> APKAPADGLKMEATKQPVVFNHSTHKSVKCGDCHHPVNGKEDYRKCGTAGCHDSMDKKDKSAKGYYHVMHDKNTKFKSCVG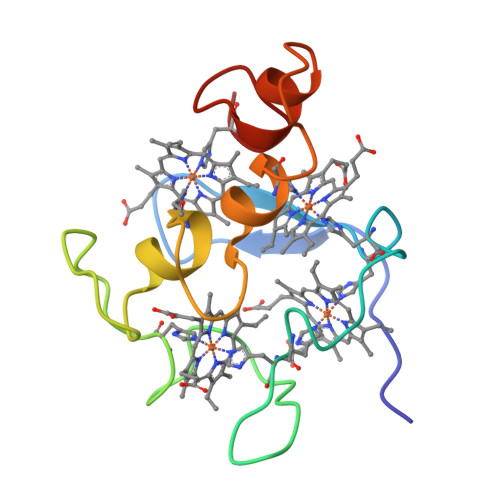CHVEVAGADAAKKKDLTGCKKSKCHE> KQDT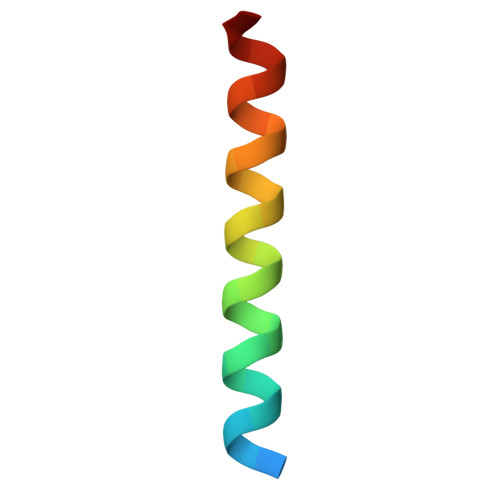ASKMKLLKKKIEEQREILQKTHHKN In the methanogenic pathway from H2 and CO2, the membrane-spanning methyl-tetrahydromethanopterin (CH3-H4MPT):coenzyme M (CoM-SH) methyltransferase complex (MtrA–H) catalyses the exergonic methyl transfer from CH3-H4MPT to CoM-SH (ΔG°′ = −30 kJ/mol) coupled with endergonic sodium-ion gradient formation. The only prosthetic group required for catalysis is vitamin B12 (cobalamin) bound to MtrA. Here, we report on the X-ray structures of the B12-binding domain of membrane-associated MtrA from Methanocaldococcus jannaschii and of the MtrA homologue from M. fervidus in complex with cobalamin. Analyses of these structures reveal a cobalamin-binding site that differs from other B12-binding proteins in an unexpected manner and also provides initial hints of how the energy of cobalt demethylation is transformed into conformational energy used for the ultimate sodium-ion translocation process.

Genome analysis has revealed an extra copy or copies of the mtrA gene in many methanogenic archaea (e.g., M. marburgensis, Methanobacterium formicicum, Methanobrevibacter ruminantium, Methanothermus fervidus and Methanosarcina barkeri). These cytoplasmic MtrA homologues consist only of a soluble cobalamin-binding domain of 170–180 amino acids, which is in contrast to the approximately 250 amino acids of membrane-associated MtrA. Crystal structures of two MtrA variants revealed a detailed view of a novel binding site for cobalamin inside a Rossmann-type domain compared with all other Rossmann-type B12 enzymes studied so far. Nevertheless, several functionally characteristic features were designed in an equivalent manner. They include an exposed corrinoid ring at the top of loops at the C-terminal side of the central β-sheet, an elongated conformation of cobalamin with the nucleotide tail between the β-sheet–α-helix layer, albeit on opposite sides, and a His-Glu-proton donor linkage on the lower axial side of the corrinoid ring. The structure of cytoplasmic MtrA complexed with cobalamin and the structure of the soluble domain of MtrA without cobalamin were essentially identical. This finding suggested that the MtrA structures observed in this work were relaxed forms. The possible repellent effect of cob(I)alamin towards the histidine residue probably causes a conformational change in the MtrA protein structure 11329. From there, the conformational changes could be transmitted further for sodium-ion transport across the cytoplasmic membrane.

>[2x]MVKKKEPAEGWPVVSGDYIVGDPESPVAAVTLASHIEDIPIDAGAAIAGPCKTENLGIEKVIANIISNPNIRFLVLCGSEVQGHIVGQSMKALHKNGVDDKRKIIGAKGAIPYIENLPEEALERFQKQVEIVDLIDVEDADQIKEKVKECIEKDPGAFEEEEVILRL;> GSHMVKKKEPAEGWPVVSGDYIVGDPESPVAAVTLASHIEDIPIDAGAAIAGPCKTENLGIEKVIANIISNPNIRFLVLCGSEVQGHIVGQSMKALHKNGVDDKRKIIGAKGAIPYIENLPEEALERFQKQVEIVDLIDVEDADQIKEKVKECIEKDPGAFEEEEVILRL> HMQHITVRLPKKARAMIVGEITNVFKDKYPIADKLKVIPEYDVIEQDLCKLLSPGFPKQPLRVYKFGSRITGIGNRSSDLDLFVDIGNTFHTFEHRASNATVAKLRAMRKFFCDSEDWRLINFI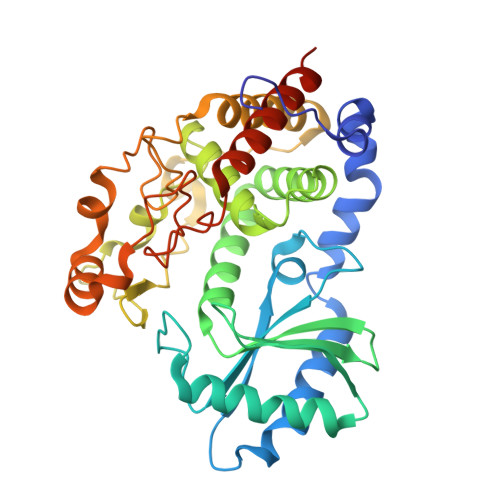EQARVPIIKTCHLPTGIECDICLNSMGFCNTNLLKYIFESQPLTQYMCIYVKNWLERCKLTEQISTYSITLMVIYFLQLQALLPPIAMLQIEDAANQAVLVGPWVVNFAQKSFSELGLQQLKATVPVIKGFLRNFFAYFAKFDYEHFLVCPYIGQANVEIAKIERMLHARYSAYVSDNPECSIQLKKPMVVQDPIQLNHNVTKAVTKYGLQTFVDYCQQTAELLEEPSTNWRQRYAF> KVVKFSYMWTINNFSFCREEMGEVIKSSTFSSGANDKLKWCLRVNPKGLDEESKDYLSLYLLLVSCPKSEVRAKFKFSILNAKGEE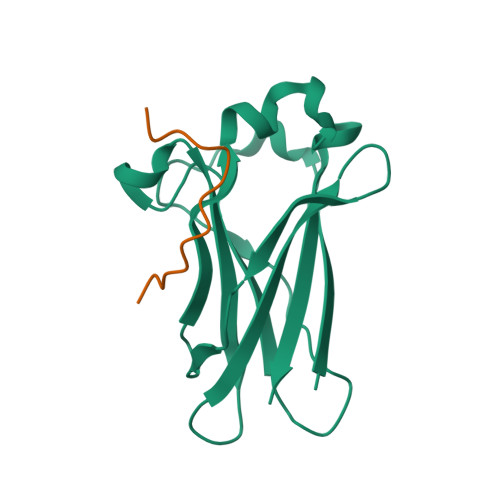TKAMESQRAYRFVQGKDWGFKKFIRRDFLLDEANGLLPDDKLTLFCEVSVVQD;> NDDDVQKADVSSTGQGV> ANSLEPEPWFFKNLSRKDAERQ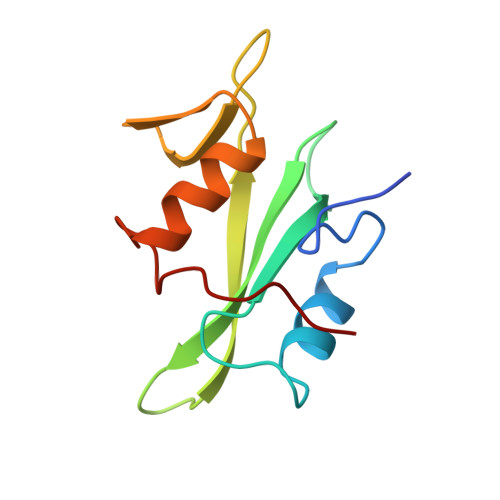LLAPGNTHGSFLIRESESTAGSFSLSVRDFDQNQGEVVKHYKIRNLDNGGFYISPRITFPGLHELVRHYTNASDGLCTRLSRPCQT>[2x]GAMETPVKIPIL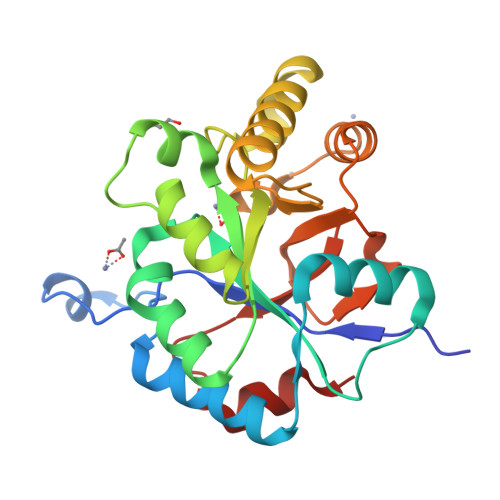MYHAIHVMSPEETANANLIVNPDLFDQQLQKMKDEGYYFLSPEEVYRALSNNELPAKKVVWLTFDDSMIDFYNVAYPILKKYDAKATNNVITGLTEMGSAANLTLKQMKEMKQVGMSFQDHTVNHPDLEQASPDVQTTEMKDSKDYLDKQLNQNTIAIAYPSGRYNDTTLQIAARLNYKLGVTTNEGIASAANGLLSLNRIRILPNMSPENLLQTMEP> MQVTHSMPPQKLEIFKSLDDWARNNVLIHLKSVEKSWQPQDYLPDPVSDGFEEQVRELRERAKEIPDDYFVVLVGDMITEEALPTYMSMLNRCDGIKDETGAEPSAWAMWTRAWTAEENRHGDLLN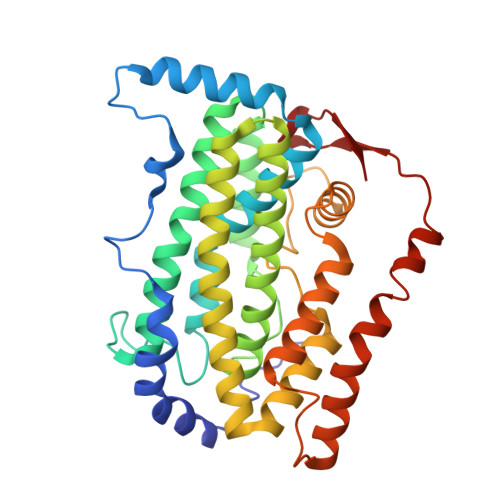KYLYLSGRVDMRKIEKTIQYLIGSGMDIKSENSPYLGFIYTSFQERATFISHANTAKLAQHWGDKNLAHICGSIASDEKRHATAYTKIVEKLAEIDPDTTVIAFADMMRKKITMPAHLMYDGSDELLFKHFTAVAQRVGVYSALDYCDILEFLVDKWNVERLTGLSDEGRKAQEYVCELGPKIRRLEERAQGRAKEAPTMPFSWIFDRQVKL(1R,2R)-cyclohexane-1,2-diol | C6 H12 O2 | 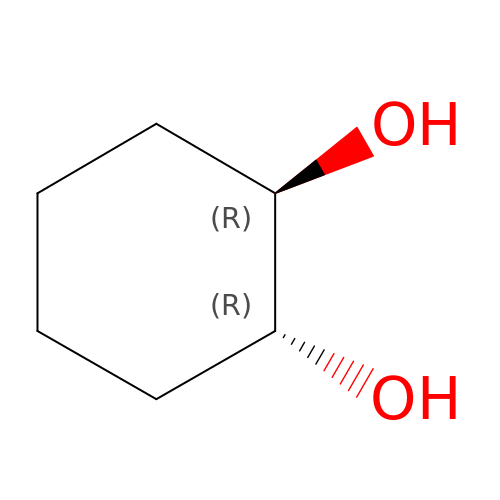PFURGBBHAOXLIO-PHDIDXHHSA-N> S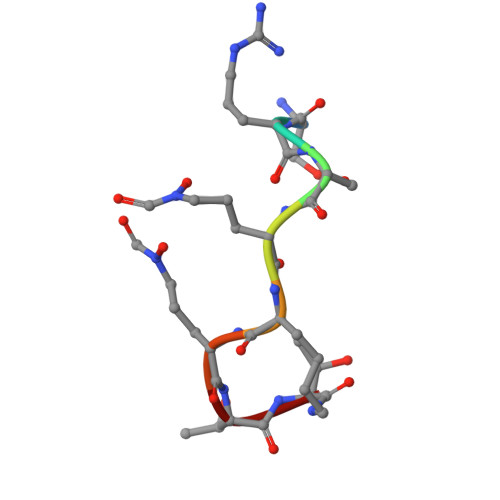RSKKKTT(3~{a}~{R},4~{S},6~{a}~{R})-1-methyl-4,5,6,6~{a}-tetrahydro-3~{a}~{H}-pyrrolo[3,4-c]pyrazole-3,4-dicarboxylic acid | C8 H11 N3 O4 | 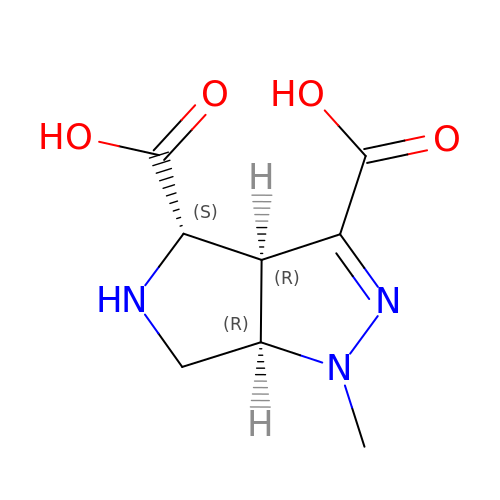MUCHMWUQFYVYSF-YUPRTTJUSA-N Thus, U6 recruitment into spliceosomes proceeds though a novel, and poorly understood, RNA remodeling mechanism involving large-scale conformational changes. The core region of the U6 snRNP retains the unique “interlocked rings” topology of Prp24 and U6 snRNA and is virtually identical to previously determined structures of U6/Prp24 binary complexes, with a comparative r.m.s.d of ~1.3 Å. There are protein–protein contacts in the U6 snRNP that were not visible in previous structures, including a 660 Å2 contact between RRM4 of Prp24 and Lsm2, and a contact between the conserved C-terminus (or “SNFFL box”) of Prp24 and Lsm5 and Lsm7. The architecture of the free U6 snRNP provides insights into how spliceosomal RNAs can be remodeled in the absence of an ATP-dependent helicase.

In order to elucidate the basis for this selectivity, we generated U6 snRNPs with 3′ terminal phosphate groups. We also used RNAs with either four or five 3′ uridines to probe the structural effect of 3′ length heterogeneity inherent to S. cerevisiae U6 snRNA12. Nucleotides between the telestem and 3′ oligouridylate tail are poorly resolved due to an apparent lack of protein-RNA contacts, which likely affords a degree of flexibility to accommodate the 3′ length heterogeneity of U6 snRNA12. Inside the ring, RNA is bound in a shifted register relative to that observed previously. Instead of being bound in the Sm-like pocket of Lsm3, the terminal nucleotide occupies a new pocket comprised of residues in Lsm2, Lsm3 and Lsm8, and the penultimate nucleotide is bound in the previously identified Sm-like pocket of Lsm3. In this new “Up” (or uridine phosphate) pocket, Lsm2 residue K20 forms a cation–pi interaction with the terminal uracil and a buried salt bridge with Lsm3 residues D71 and R69, the latter of which participates in a cation–pi interaction with the penultimate uracil. The remaining contacts with the terminal uridylate are dominated by electrostatic interactions with Lsm3-R21 and Lsm8-K87, K90 and K92.

> MKKANEALTRNRELTTVLVKNLPKSYNQNKVYKYFKHCGPIIHVDVADSLKKNFRFARIEFARYDGALAAITKTHKVVGQNEIIVSHLTECTLWMTNFPPSYTQRNIRDLLQDINVVALSIRLPSLRFNTSRRFAYIDVTSKEDARYCVEKLNGLKIEGYTLVTKVSNPLEKSKRTDSATLEGREIMIRNLSTELLDENLLRESFEGFGSIEKINIPAGQKEHSFNNCCAFMVFENKDSAERALQMNRSLLGNREISVSLADKKPFLERNEVKRLLASRNSKELETLICLFPLSDKVSPSLICQFLQEEIHINEKDIRKILLVSDFNGAIIIFRDSKFAAKMLMILNGSQFQGKVIRSGTINDMKRYYNNQQNHSMKHVKPSCINMMEKGPNLQVKKKIPDKQEQMSNDDFRKMFLGEHHHHHH;> MLFFSFFKTLVDQEVVVELKNDIEIKGTLQSVDQFLNLKLDNISCTDEKKYPHLGSVRNIFIRGSTVRYVYLNKNMVDTNLLQDATRREVMTERK;> METPLDLLKLNLDERVYIKLRGARTLVGTLQAFDSHCNIVLSDAVETIYQLNNEELSESERRCEMVFIRGDTVTLISTPSEDDDGAVEIWSHPQFEK;> MLPLYLLTNAKGQQMQIELKNGEIIQGILTNVDNWMNLTLSNVTEYSEESAINSEDNAESSKAVKLNEIYIRGTFIKFIKLQDNIIDKVKQQI;> MSLPEILPLEVIDKTINQKVLIVLQSNREFEGTLVGFDDFVNVILEDAVEWLIDPEDESRNEKVMQHHGRMLLSGNNIAILVPGGKKTPTEAL;> GSMSGKASTEGSVTTEFLSDIIGKTVNVKLASGLLYSGRLESIDGFMNVALSSATEHYESNNNKLLNKFNSDVFLRGTQVMYISEQKI;> MHQQHSKSENKPQQQRKKFEGPKREAILDLAKYKDSKIRVKLMGGKLVIGVLKGYDQLMNLVLDDTVEYMSNPDDENNTELISKNARKLGLTVIRGTILVSLSSAEGSDVLYMQK;> MSATLKDYLNKRVVIIKVDGECLIASLNGFDKNTNLFITNVFNRISKEFICKAQLLRGSEIALVGLIDAENDDSLAPIDEKKVPMLKDTKNKIENEHVIWEKVYESKTKHHHHHH>GSKGVSDLLGFKIFGMPLPLYAFALITLLLSHFYNALPTDIVGGFAIMFIIGAIFGEIGKRLPIFNKYIGGAPVMIFLVAAYFVYAGIFTQKEIDAISNVMDKSNFLNLFIAVLITGAILSVNRRLLLKSLLGYIPTILMGIVGASIFGIAIGLVFGIPVDRIMMLYVLPIMGGGNGAGAVPLSEIYHSVTGRSREEYYSTAIAILTIANIFAIVFAAVLDIIGKKHTWLSGEGELVRKASFKVEEDEKTGQITHRETAVGLVLSTTCFLLAYVVAKKILPSIGGVAIHYFAWMVLIVAALNASGLCSPEIKAGAKRLSDFFSKQLLWVLMVGVGVCYTDLQEIINAITFANVVIAAIIVIGAVLGAAIGGWLMGFFPIESAITAGLCMANRGGSGDLEVLSACNRMNLISYAQISSRLGGGIVLVIASIVFGMMIPR[4x]

The 2-HCT family of transporters generally translocate molecules with a 2-hydroxycarboxylate motif (HO-CR1R2-COO−), such as citrate, malate and lactate across the plasma membrane, and activity is tightly coupled to energy provided by a sodium or proton gradient as a form of secondary active transport. Our crystal structures reveal that the KpCitS protomer is formed by homologous N-terminal and C-terminal halves with inverted topology, each containing six transmembrane helices (TM 2–5, 7 and TM 8–11, 13) and one helical hairpin (TM 6a/b (or HP1) and TM 12a/b (or HP2)). KpCitS protomer can be divided into two domains; a central dimerization domain (TM 1–4 and 8–10) critical for formation of the dimeric structure, and a peripheral transport domain (TM 5–7 and 11–13) containing residues needed for interaction with citrate and sodium ions. Our results show that the KpCitS has a homodimeric structure in which its dimerization domain remains fixed during the transport cycle due to a hydrogen bond network as well as extensive hydrophobic interactions, while the substrate-loaded transport domain undergoes an elevator-type translocation (i.e. up and down) across the membrane.

The final models showed that two crystal forms of KpCitS were obtained in the citrate-containing droplet. In contrast, the other crystal form (form 2), refined to 3.8 Å resolution, contains two pairs of KpCitS dimers in an asymmetric unit; one has an outward-facing conformation, and the other an asymmetric conformation. For the sake of the accuracy, we selected the structure of the highest resolution dataset from each of the three major conformational states for analysis; thus, the outward-facing, inward-facing, and asymmetric conformations of crystal forms 2, 3, and 4, respectively, are shown throughout this article. In the outward-facing state, the hairpin loops are located close to the membrane/periplasm interface, which appears to favor the entry of external substrate and ions (left). In the outward-facing state the bound citrate is partially exposed to the periplasmic space. However, it is unlikely that it can escape backwards because it is secured by strong hydrogen and electrostatic interactions. In the outward-facing conformation, L408 and I121 are in close proximity, and serve as a latch governing access of substrate to the cytoplasm. In addition, M417 seems to act as a plug preventing substrate exit.>MFTGSIVAIVTPMDEKGNVCRASLKKLIDYHVASGTSAIVSVGTTGESATLNHDEHADVVMMTLDLADGRIPVIAGTGANATA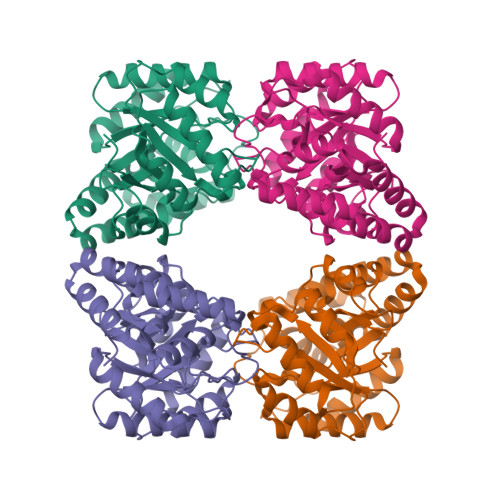EAISLTQRFNDSGIVGCLTVTPYYNRPSQEGLYQHFKAIAEHTDLPQILFNVPSRTGCDLLPETVGRLAKVKNIIGIKEATGNLTRVNQIKELVSDDFVLLSGDDASALDFMQLGGHGVISVTANVAARDMAQMCKLAAEGHFAEARVINQRLMPLHNKLFVEPNPIPVKWACKELGLVATDTLRLPMTPITDSGRETVRAALKHAGLL[2x]> GAMGSEKSPSAQELKEQGNRLFVGRKYPEAAACYGRAITRNPLVAVYYTNRALCYLKMQQHEQALADCRRALELDGQSVKAHFFLGQCQ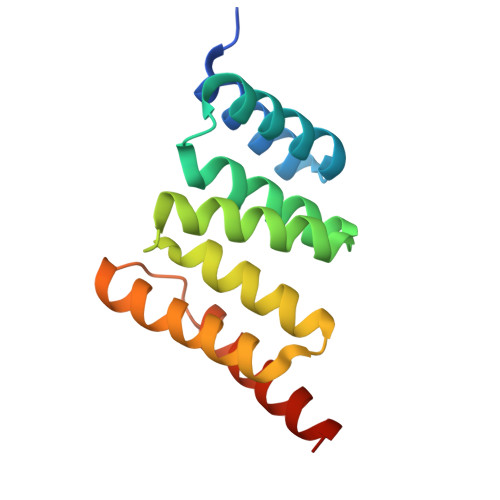LEMESYDEAIANLQRAYSLAKEQRLNFGDDIPSALRIAKKKRWNSIEERR> MSTNKVNKERTFLAVKPDGVARGL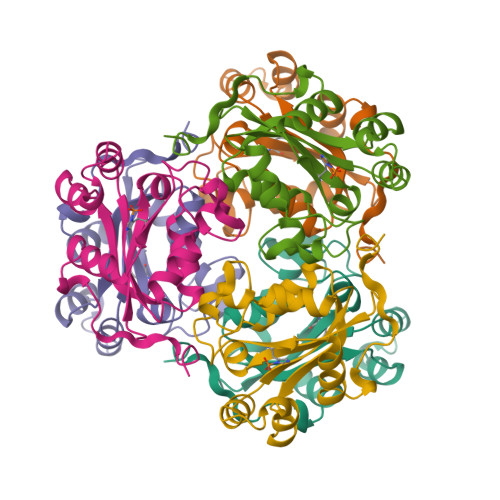VGEIIARYEKKGFVLVGLKQLVPTKDLAESHYAEHKERPFFGGLVSFITSGPVVAMVFEGKGVVASARLMIGVTNPLASAPGSIRGDFGVDVGRNIIHGSDSVESANREIALWFKPEELLTEVKPNPNLYE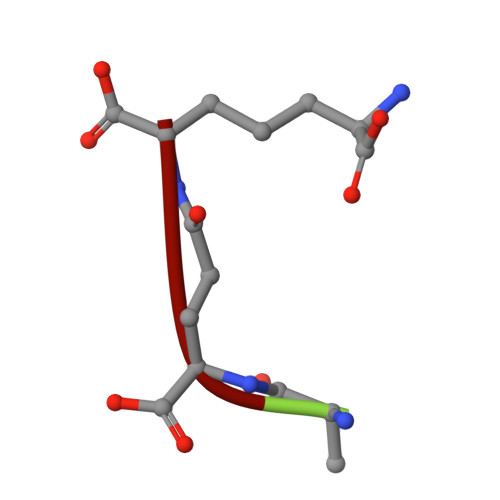> AEK> MHHHHHHGGGGGMINKPNQFVNHLSALKKHFASYKELREAFNDYHKHNGDELTTFFLHQFDKVMELVKQKDFKTAQSRCEEELAAPYLPKPLVSFFQSLLQLVNHDLLEQQNAALASLPAAKIIELVLQDYPNKLNMIHYLLPKTKAFV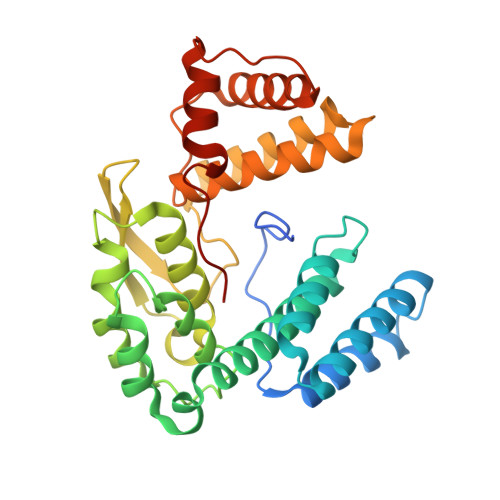KPHLLQRLQFVLTDSELLELKRFSFFQALNQIPGFQGEQVEYFNSKLKQKFTLTLGEFEIAQQPDAKAYFEQLITQIQQLFLKEPVNAEFANEIIDAFLVSYFPLHPPVPLAQLAAKIYEYVSQIVLNEAVNLKDELIKLIVHTLYEQLDRPVGDEN>MAHHHHHHVFFAVITLFPEMFDAITAYGISGRAAKRDIVQVTCINPRDFAEGNYRRVDERPFGGGPGMVMMAEPLAKAINHAKQLASRAGCVHVPVVYMSPQGKTLNEQAVQQFVDYDGLIVLCGRYEGVDERLIQHYVDQEWSIGDYVLSGGELPAMVLLDSIIRRLPNVMSDEQSAIQDSFVDGLLDCPQYTKPDQFEGLDVPEILKSGHHANIEKWRFLQ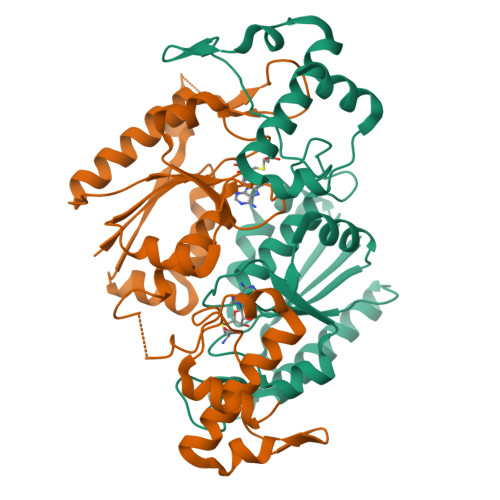RYQRTLERRPELIEQVTLTKQQKKWLSDEQG[2x]>GSMSIKSDKWIRRMAEEHKMIEPFVPDQVRAAEDGRRIVSYGTSSYGYDIRCADEFKIFTNINSTIVDPKNFDEGSFVDFKGDVCIIPPNSFALARTVEYFRIPRTVLTVCLGKSTYARCGIIVNVTP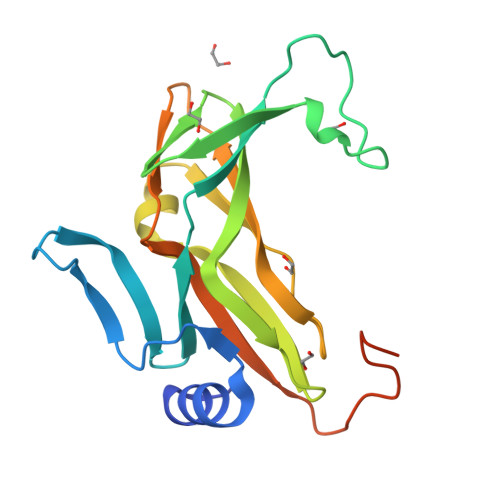FEPEWEGYVTLEFSNTTPLPAKIYANEGVAQVLFFESDEVCDVSYADRGGKYQGQRGVTLPKT[2x]>[4x]MDSTKAQTPEEQRAKNAKTILENIQIYERMCDLFGVSEDDKLIIENSISIERMIRVVTDKKYQDKKLKNAGSDPEKIANAGKVFCRLVESTAGKCSARLGMALKPNVEAVLTDVLGNELDRAAVLGKRMGFSAMFKSNLEEVLYQRGKNQLKKRNAAETFTLSQGASLEARFRPIMEKHLGVGTVVASIKNILASKKNGNYRNKMVRKPGGNRESWSPLEREISFLNKKLFPGPMRQLCKKFEYLNEQEKQLALNLMLDASLILKPQVTHK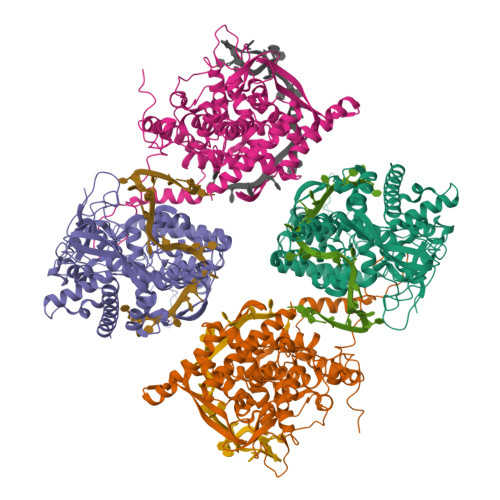MIMPWSMWLAVKKYAEMNKGSPSLEDLAAYSGVRAFMAFNTACYMSKFTIGKGIVGDAEIMENGNDKMQTLAMACFGLAYEDTGIVAAMISQPMKKRYQLRVGNFNPPEKGTIKGTSAGYFHKWAEFGNRLPFNSFGTGESKQISNSGVFAVQRPSTTNIQRLAELMARNTGETSDNFTQLVQKIREQVGAFADQKANLREFTGGYIYDITDVTKSNPKIPQLGGDSFFFEFTGSDVPRTGAKRRVGGADDVTPGTSQPKKRGRQGAGAESSMDIETVGED> MQGSVTEFLKPRLVDIEQVSSTHAKVTLEPLERGFGHTLGNALRRILLSSMPGCAVTEVEIDGVLHEYSTKEGVQEDILEILLNLKGLAVRVQGKDEVILTLNKSGIGPVTAADITHDGDVEIVKPQHVICHLTDENASISMRIKVQRGRGYVPASTRIHSEEDERPIGRLLVDACYSPVERIAYNVEAARVEQRTDLDKLVIEMETNGTIDPEEAIRRAATILAEQLEAFVDLE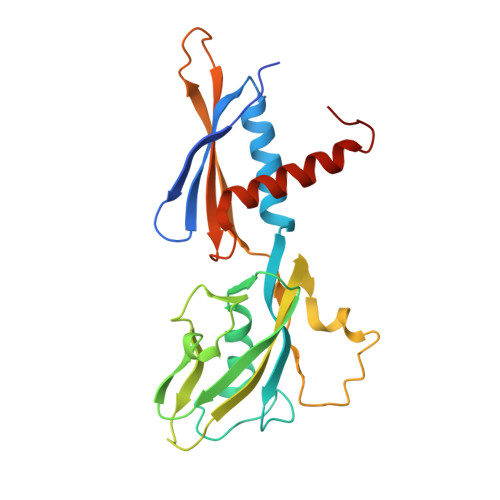VLF>[2x]MPVLENRAAQGDITAPGGARRLTGDQTAALRDSLSDKPAKNIILLIGNGMGDSEITAARNYAEGAGGFFKGIDALPLTGQYTHYALNKKTGKPDYVTDSAASATAWSTGVKTYNGALGVDIHEKDHPTILEMAKAAGLATGNVSTAELQDATPAALVAHVTSRKCYGPSATSEKCPGNALEKGGKGSITEQLLNARADVTLGGG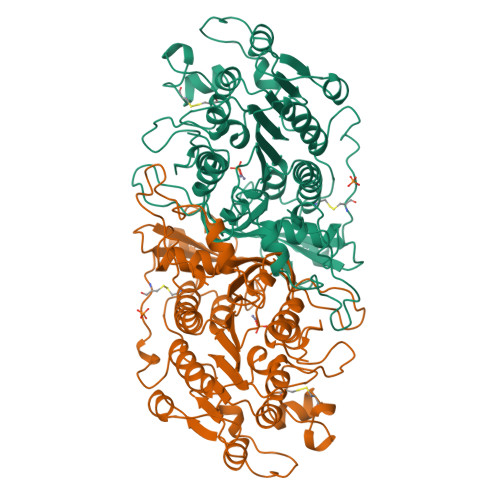AKTFAETATAGEWQGKTLREQAQARGYQLVSDAASLNSVTEANQQKPLLGLFADGNMPVRWLGPKATYHGNIDKPAVTCTPNPQRNDSVPTLAQMTDKAIELLSKNEKGFFLQVEGASIDKQDHAANPCGQIGETVDLDEAVQRALEFAKKEGNTLVIVTADHAHASQIVAPDTKAPGLTQALNTKDGAVMVMSYGNSEEDSQEHTGSQLRIAAYGPHAANVVGLTDQTDLFYTMKAALGLK> MEKTYNLNDILLSNEYEKIKEDIKEEIINDMASKKVKYSNTSEFAKNDFLKDEFIDLVVDGETYEITYGNLITLLIVARPFNHFKVPMTEDLLFDLSDLKEYQNYYTTLLEHFGYSNEIKSIIKDVISELAIFSGDINVTFGNTVSIKSLIDLGNKVKRFRELLHYRLPNDEALEFNDIEAIIKKNLDEIMKILSETDNMLRYYIDSGAGINSKQFGQVLSLVGSKPDLFGKIIPYPINTSFLRGLDVRSFYINALGARKALITNYQQVRNSGYLTRKISMLLMDTKLIDLDDCGSHENNYLSINVENKDVLKRFSKRSYLNNNGELVEIDINDESLIGQVIKIPSPTTCASNEGVCRKCYGKLFDINKDLNIGMIAVLLLTDPLTQRLLSAKHLLETRSSKIDWGTNFEENFIVNRNLIYPKVYNGTVIIKEDDFKEDEET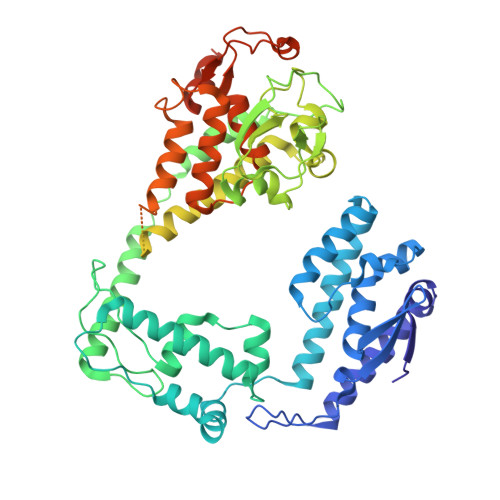EEQVFDTFTLKSGNRFISISSPMRLFLNKDLKKQLDESFYNIEEMQFEIPLNKLDEGDSFATFIMDNNELSKPLREIKDLIETNKYIKDHNVNEVVNYFIYLLNESGINIQSVHSELIIREMMKLDDSDRTQFKNDKMPDYEIFRITDANLKGDSLSRSLLFEQVKKQLTTLDYDTFNKTKSSILDKLL Unlike other PLs, Smlt1473 present in the clinically relevant Stenotrophomonas maltophilia strain K279a demonstrates a wide range of pH-dependent substrate specificities toward multiple, diverse polysaccharides: hyaluronic acid (pH 5.0), poly-β-D-glucuronic (celluronic) acid (pH 7.0), poly-β-D-mannuronic acid, and poly-α-L-guluronate (pH 9.0). To decode the pH-driven multiple substrate specificities and selectivity in this single enzyme, we present the X-ray structures of Smlt1473 determined at multiple pH values in apo and mannuronate-bound states as well as the tetra-hyaluronate-docked structure. We have built and refined the structures from residues A22-L330; electron density for other residues outside this range was either weak or absent. The structure is composed of 13 α-helical segments (α-1 to α-13) connected by 14 loops (L-1 to L-14) and two β-strands (β-1 and β-2) (Fig. 2, B and C (i and ii)).

In order to visualize and understand the effects of pH on Smlt1473 structure, we have crystallized and determined the protein structure at different pH values (5.0, 5.5, 6.5, 7.0, 8.5, and 9.0). The atomic superposition of all the crystal structures across the entire range of pH values did not show any significant change as a function of pH. However, significant rotameric transitions of important substrate-binding residues such as K42, K162, R163, H221, and R312L have been observed at different pH values. At the entry site, the residues involved in rotameric transition are H221 and R312, of which H221 has an altered orientation in all structures above pH 5.0, whereas R312 has an altered orientation only in the pH 7.0 structure due to a hydrogen bonding interaction with Y225. At the exit site, K42 exhibits an altered orientation only in the pH 6.5 and 9.0 structures, whereas in pH 5.0 and pH 5.5 there is no change in orientation; interestingly, at pH 7.0 and 8.5 a lack of electron density precluded analysis of the residue orientation. For K162, the altered orientation was observed only for the pH 6.5 and 9.0 structures; for pH 7.0 and pH 8.5 a lack of electron density precluded analysis of residue orientation.

>ACPAPPPGQPDIRAIGYYTDKAGSVIDPALQQQNKDATAPLDRYAADVARMSDDYLRNGDPAAAQCTLSWLGAWADDGAMLGQMIRVNNDQSFYMRQWMLDAVAMAYLKVHDQANPQQRARIDPWLQKLARANLAYWDNPKRRRNNHYYWGGLGVLATGLATDDDALWQAGHAAFQKGIDDIQDDGSLPLEMARGQRALHYHDYALAPLVMMAELARLRGQDWYASRNHAIDRLARRVIEGSRDPAWFNQHTGAAQLPLQASGWVEFYRLRSPDGGVFDAAHARGPFHSPRLGGDLTLMATHGIVRTPLRHHHHHH[2x]> QYYREGTGSYTVVLPPGAKVPQAEIYKTSNLQGAVPTNSWESSILWNQYSLPIYAHPLTFKFKAEGIEVGKPALGGSGIAYFGAHKNDFTVGHSSVYTFPDARADKISDFAVDAVMASGSGSIKATLMKGSPYAYFVFTGGNPRIDFSGTPTVFYGDSGSQCLGVTINGVNYGLFAPSGSKWQGIGTGTITCILPAGKNYFSIAVLPDNTVSTLTYYKDYAYCFVTDTKVEWSYNETESTLTTTFTAEVSVKEGTNKGTILALYPHQWRNNPHILPLPYTYSTLRGIMKTIQGTSFKTVYRYHGILPNLPDKGTYDREALNRYINELALQADAPVAVDTYWFGKHLGKLSCALPIAEQLGNISAKDRFISFMKSSLEDWFTA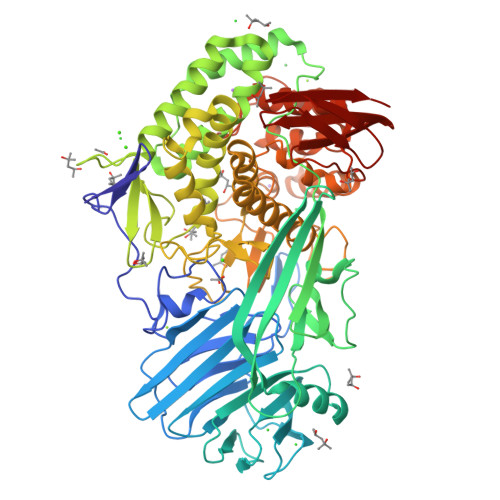KEGETAKLFYYDSNWGTLIGYPSSYGSDEELNDHHFHYGYFLHAAAQIALRDPQWASRDNWGAMVELLIKDIANWDRNDTRFPFLRNFDPYEGHSWASGHAGFADGNNQASSSEAINAWQAIILWGEATGNKTIRDLGIYLYTTEVEAVCNYWFDLYKDIFSPSYGHNYASMVWGGKYCHEIWWNGTNSEKHGINFLPITAASLYLGKDPNYIKQNYEEMLRECGTSQPPNWKDIQYMYYALYDPAAAKNMWNESIVPEDGESKAHTYHWICNLDSLGLPDFSVTADTPLYSVFNKNNIRTYVVYNASSSAKKVTFSDGKVMTVGPHSMAVSTGS>IPCGESCVWLPCISSAIGCSCKSKVCYRNG[2x]

Cyclotides are a large family of topologically unique peptides characterized by a head-to-tail cyclic backbone and three interlocked disulfide bonds. This combination of structural features forms a cyclic cystine knot (CCK) motif and confers cyclotides exceptional stability. Cyclotides are divided into three subfamilies: bracelet, Möbius, and trypsin inhibitor subfamilies. Since cyclotides were first reported two decades ago, studies on bracelet cyclotides have been hampered by their low synthetic yields because of poor oxidative folding efficiency.

Since Ile-11 appears to be critical for folding of bracelet cyclotides, it was of interest to explore the capacity of this position to tolerate another branched residue, Leu. Surprisingly, the four [I11L] mutants exhibited yields from 13%–44%, which is lower than that of the [I11G] mutants but still substantially higher than that obtained from the native parent peptides. When the Ile was mutated to Leu instead, bioactivity was retained. Contrary to the [I11G] results, the [I11L] mutants exhibited equipotent binding to the POPC/POPE (80:20) model membrane compared to their wild-type counterparts. [I11L] mutants exhibited similar or slightly higher cytotoxicity compared to their parent cyclotides, whereas the [I11G] mutants had substantially reduced or no activity, which correlates well with their membrane binding. Overall, these results confirmed that the [I11L] mutants retain the biological properties of their native bracelet cyclotides. Using this I11L mutation, we synthesized all d-enantiomers of I11L mutants of bracelet cyO2 from Viola odorata and bracelet hyen D from Hybanthus enneaspermus. Having determined the crystal structures of wild-type cyO2 and hyen D, we were interested in definitively showing their Ile-11 to Gly and Leu mutants have native-like structures to support our earlier NMR chemical shift analysis. Their structures were solved using racemic or quasi-racemic crystallography.>[7x]SNAAKDVKFGADARALMLQGVDLLADAVAVTMGPKGRTVIIEQSWGSPKVTKDGVTVAKSIDLKDKYKNIGAKLIQDVANNTNEEAGDGTTTATVLARSIAKEGFEKISKGANPVEIRRGVMLAVDAVIAELKKQSKPVTTPEEIAQVATISANGDKEIGNIISDAMKKVGRKGVITVKDGKTLNDELEIIEGMKFDRGYISPYFINTSKGQKCEFQDAYVLLSEKKISSIQSIVPALEIANAHRKPLVIIAEDVDGEALSTLVLNRLKVGLQVVAVKAPGFGDNRKNQLKDMAIATGGAVFGEEGLTLNLEDVQPHDLGKVGEVIVTKDDAMLLKGKGDKAQIEKRIQEIIEQLDVTTSEYEKEKLNERLAKLSDGVAVLKVGGTSDVEVNEKKDRVTDALNATRAAVEEGIVLGGGCALLRCIPALDSLTPANEDQKIGIEIIKRTLKIPAMTIAKNAGVEGSLIVEKIMQSSSEVGYDAMAGDFVNMVEKGIIDPTKVVRTAL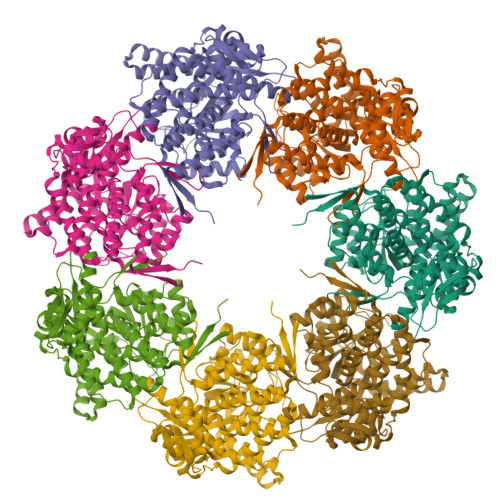LDAAGVASLLTTAEVVVTEIPKEEKDPGMGAMGGMGGGMGGGMF>[2x]MEEGGST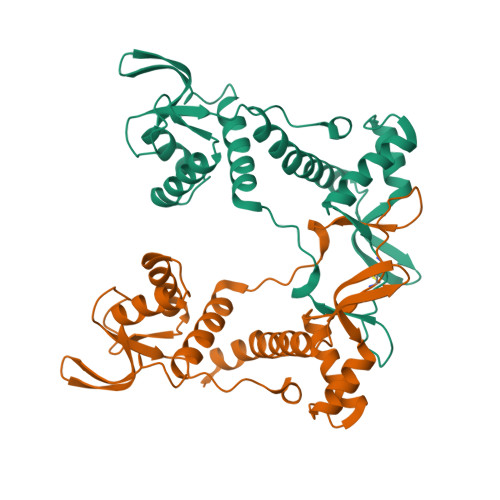GSAGSDSSTSGSGGAQQRELERMAEVLVTGEQLRLRLHEEKVIKDRRHHLKTYPNCFVAKELIDWLIEHKEASDRETAIKLMQKLADRGIIHHVCDEHKEFKDVKLFYRFRKDDGTFPLDNEVKAFMRGQRLYEKLMSPENTLLQPREEEGVKYERTFMASEFLDWLVQEGEATTRKEAEQLCHRLMEHGIIQHVSSKHPFVDSNLLYQFRMNFRRRRRLMEL> MSYQGRARKFLESASIDVGDMVLVEKPDVTYEGMVLDRADDADDRHIVLKLENGYNIGVEISDARIELLEKGSEPRIELPPVEAAEDPELPDVSIISTGGTVASIIDYRTGAVHPAFTADDLLRANPELLDIANIRGRAVFNILSENMKPEYWVETARAVYGEIKDGADGVVVAHGTDTMHYTSAALSFMLRTPVPVVFTGAQRSSDRPSSDASLNIQ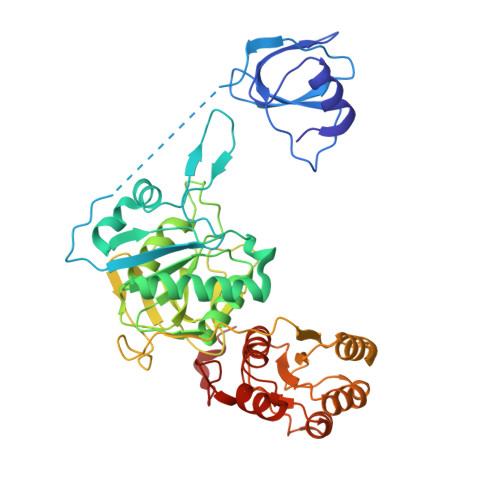CSVRAATSEIAEVTVCMHATMDDLSCHLHRGVKVRKMHTSRRDTFRSMNALPLAEVTPDGIKILEENYRKRGSDELELSDRVEERVAFIKSYPGISPDIIKWHLDEGYRGIVIEGTGLGHCPDTLIPVIGEAHDMGVPVAMTSQCLNGRVNMNVYSTGRRLLQAGVIPCDDMLPEVAYVKMCWVLGQTDDPEMAREMMRENIAGEINERTSIAYFRG>[2x]DSGCVVSWKNKELKCGSGIFITDNVHTWTEQYKFQPESPSKLASAIQKAHEEGICGIRSVTRLENLMWKQITPELNHILTENEVKLTIMTGDIKGIMQAGKRSLRPQPTELKYSWKAWGKAKMLSTELHNHTFLIDGPETAECPNTNRAWNSLEVEDYGFGVFTTNIWLKLKERQDVFCDSKLMSAAIKDNRAVHADMGYWIESALNDTWKIEKASFIEVKSCHWPKSHTLWSNGVLESEMIIPKNFAGPVSQHNYRPGYHTQTAGPWHLGRLEMDFDFCEGTTVVVTEDCGNRGPSLRTTTASGKLITEWCCRSCTLPPLRYRGEDGCWYGMEIRPLKEK

NS1 is secreted alongside dengue virus particles during an infection. It is a multifunctional protein which exists in different oligomeric forms intracellularly and extracellularly, and they play distinctly different roles. The intracellular NS1 (iNS1), exists as a membrane associated dimeric form and is a part of the viral replication complex. The extracellular secreted NS1 (sNS1), exists in higher oligomeric forms. sNS1 likely causes vascular leakage symptoms in DHF/DSS via two pathways—indirectly, by stimulating the innate immune response through activation of complement and Toll-like receptors, and directly, by binding to endothelial cells causing endothelial hyperpermeability. sNS1 when bound directly to endothelial cells causes barrier dysfunction of the cell monolayer as demonstrated in an in vitro trans-endothelial electrical resistance (TEER) assay. Here we show by cryoEM that the recombinant sNS1 exists in multiple oligomeric states: the tetrameric (stable and loose conformation) and hexameric structures.

We have also done focused refinement on one of the dimers of the loose tetramer and it is determined to 3.4 Å resolution.>[2x]HMVEFVKICGVKTMDELRLVERYADATGVVVNSRSKRKVPLKTAAELI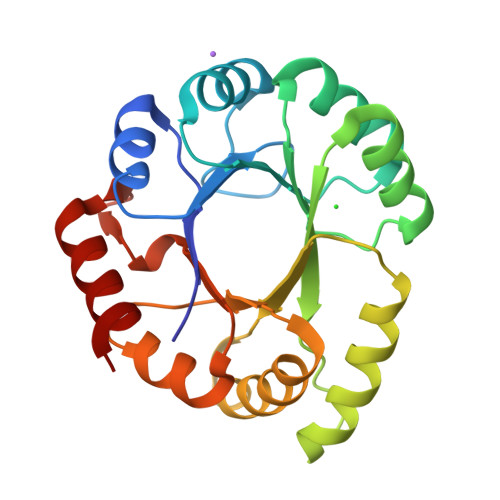EMAEIPIYLVSTMKTFPEWANAVEKTGAEYIQVHSDMHPKAVNRLKDEYGVSVMKAFMVPRESDDPAEDAERLLELIGQYEVDKILLDTGVGSGRRHDYRVSAIIAKEYPIVLAGGLTPENVGEAIRWVKPAGVDVSSGVERNGVKDRVLIEAFMAVVRNG> MPGTKRFQHVIETPEPGKWELSGYEAAVPITEKSNPLTQDLDKADAENIVRLLGQCDAEIFQEEGQALSTYQRLYSESILTTMVQVAGKVQEVLKEPDGGLVVLSGGGTSGRMAFLMSVSFNQLMKGLGQKPLYTYLIAGGDRSVVASREGTEDSALHGIEELKKVAAGKKRVIVIGISVGLSAPFVAGQMDCCMNNTAVFLPVLVGFNPVSMARNDPIEDWSSTFRQVAERMQKMQEKQKAFVLNPAIGPEGLSGSSRMKGGSATKILLETLLLAAHKTVDQGIAASQRCLLEILRTFERAHQVTYSQSPKIATLM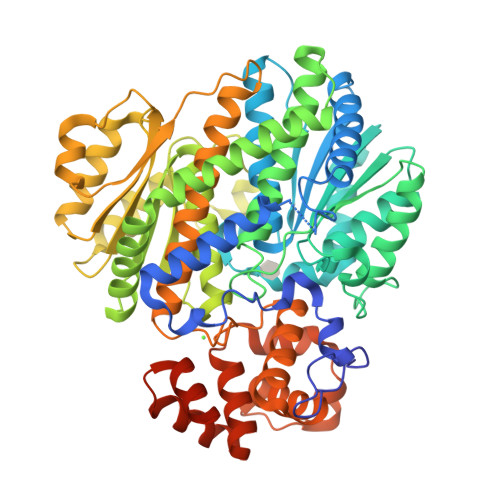KSVSTSLETTGHVYLVGWQTLGIIAIMDGVECIHTFGADFRDVRGFLIGDHSDMFNQKAELTNQGPQFTFSQEDFLTSILPSLTEIDTVVFIFTLDDNLTEVQTIVEQVKEKTNHIQALAHSTVGQTLPIPLKKLFPSIISITWPLLFFEYEGNFIQKFQRELSTKWVLNTVSTGAHVLLGKILQNHMLDLRISNSKLFWRALAMLQRFSGQSKARCIESLLRAIHFPQPLSDDIRAAPISCHVQVAHEKEQVIPIALLSLLFRCSITEAQAHLAAAPSVCEAVRSALAGPGQKRTADPLEILEPDVQLEHHHHHH>[8x]MGSSHHHYHHENLYFQGSEELYYSVEYKNTATFNKLVKKKSLNVVYNIPELHVAQIKMTKMHANALANYKNDIKYINATCSTCITSEKTIDRTSNESLFSRQWDMNKITNNGASYDD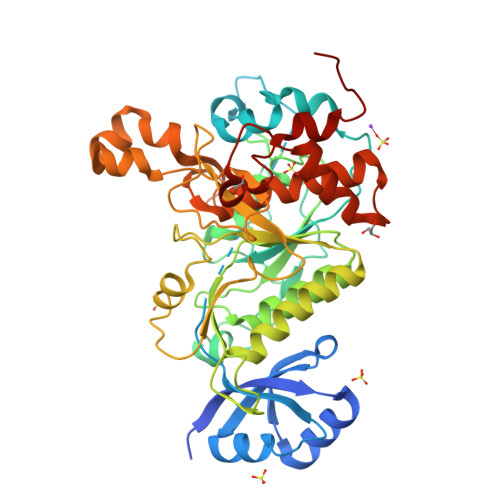LPKHANTKIAIIDTGVMKNHDDLKNNFSTDSKNLVPLNGFRGTEPEETGDVHDVNDRKGHGTMVSGQTSANGKLIGVAPNNKFTMYRVFGSKKTELLWVSKAIVQAANDGNQVINISVGSYIILDKNDHQTFRKDEKVEYDALQKAINYAKKKKSIVVAAAGNDGIDVNDKQKLKLQREYQGNGEVKDVPASMDNVVTVGSTDQKSNLSEFSNFGMNYTDIAAPGGSFAYLNQFGVDKWMNEGYMHKENILTTANNGRYIYQAGTSLATPKVSGALALIIDKYHLEKHPDKAIELLYQHGTSKNNKPFSRYGHGELDVYKALNVANQKAS> MYTSSMTYESLYTKYRDDSAILKTEDYAHWTLPTVYADPDLREGKRVNVRRDYQSVGAVYVNTLSAKLAQVLFPANQAFFRIDSTGDAAQLAEAMGAESADLANGLAELENTAFRRIFLKSSYHQLVHAMKLLIITGNVLLYRDSNTGNMHAYSIRQYSVLRDGGGKVLDMVLKERTVISELPVEARIKYRNRKQDDCICLYTRIKRERRAVGEVFVVTQQLEDGLMLDNLEVYPEAICPFIPAVWNLVTGETYGRGLVEDYAGDLAKLSALSEALALYEIEACRVLHMAKPGSQIDVDSMAERESGAWVAGDPNGVAAYEAGDYNKIIALTQEIQSIAARLAPAFMYAQNQRNAERVTAEEIRQNAEEAELALGGVYSVIADTLHIPLAHILCWEVNQQFINELLSNGLTLSVLTGVAALSRSTDVNKLIQAAQSLSVILPVFQNTPRVDPEKILDMVLTGFGINTKDLYRT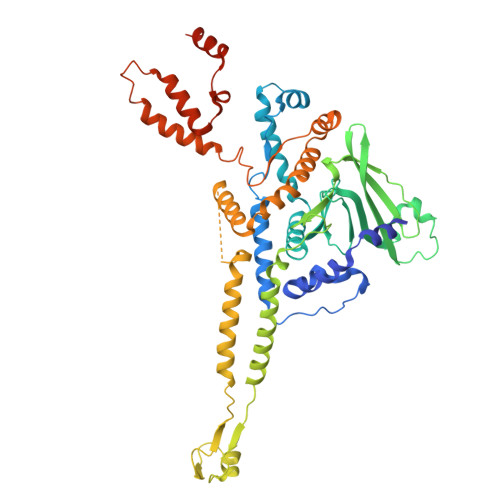EEQLQALQAAQAPVTPDLANVAGTINETGL>MSFSQAVSGLNAAATNLDVIGNNIANSATYGFKSGTASFADMFAGSKVGLGVKVAGITQDFTDGTTTNTGRGLDVAISQNGFFRLVDSNGSVFYSRNGQFKLDENRNLVNMQGMQLTGYPATGTPPTIQQGANPAPITIPNTLMAAKSTTTASMQINLNSTDPVPSKTPFSVSDADSYNKKGTVTVYDSQGNAHDMNVYFVKTKDNEWAVYTHDSSDPAATAPTTASTTLKFNENGILESGGTVNITTGTINGATAATFSLSFLNSMQQNTGANNIVATNQNGYKPGDLVSYQINNDGTVVGNYSNEQEQVLGQIVLANFANNEGLASQGDNVWAATQASGVALLGTAGSGNFGKLTNGALE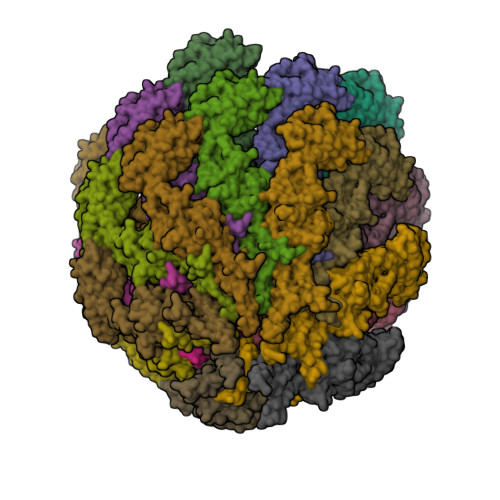ASNVDLSKELVNMIVAQRNYQSNAQTIKTQDQILNTLVNLR[22x]> GSHMSTEVDEVSALRYRIEWRPTGAGEPARLDGTWLVAKYAGTADETSTAAREALESAGARVRELVVDARCGRDELA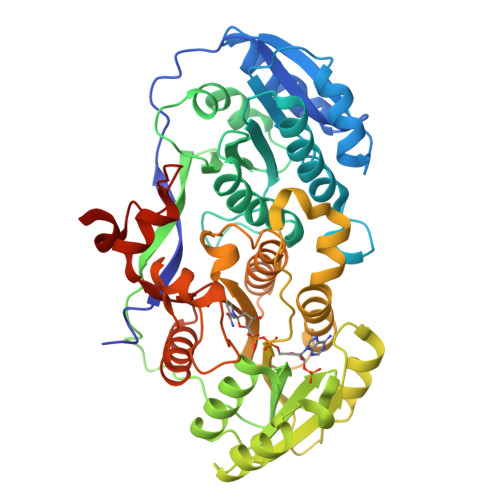ERLRSVGEVAGVLSLLAVDEAEPEEAPLALASLADTLSLVQAMVSAELGCPLWTVTESAVATGPFERVRNAAHGALWGVGRVIALENPAVWGGLVDVPAGSVAELARHLAAVVSGGAGEDQLALRADGVYGRRWVRAAAPATDDEWKPTGTVLVTGGTGGVGGQIARWLARRGAPHLLLVSRSGPDADGAGELVAELEALGARTTVAACDVTDRESVRELLGGIGDDVPLSAVFHAAATLDDGTVDTLTGERIERASRAKVLGARNLHELTRELDLTAFVLFSSFASAFGAPGLGGYAPGNAYLDGLAQQRRSDGLPATAVAWGTWAGSGMAEGPVADRFRRHGVIEMPPETACRALQNALDRAEVCPIVIDVRWDRFLLAYTAQRPTRLFDEIDDARRAAPQAAAEPR>MASPSKAVIVPGNGGGDVTTHGWYGWVKKELEKIPGFQCLAKNMPDPITARESIWLPFMETELHCDEKTIIIGHSSGAIAAMRYAETHRVYAIVLVSAYTSDLGDENERA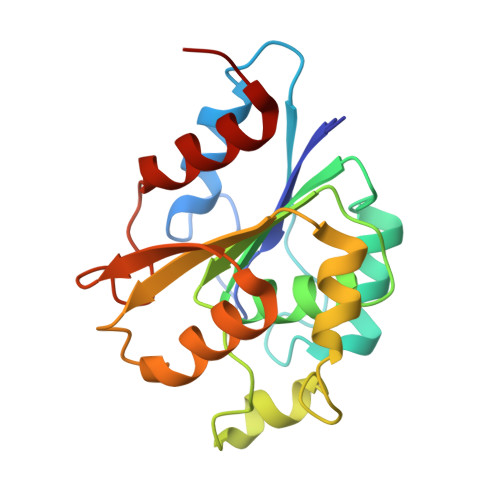SGYFTRPWQWEKIKANCPYIVQFGSTDDPFLPWKEQQEVADRLETKLHKFTDCGHFQNTEFHELITVVKSLLKVPA[2x]>MKRSWF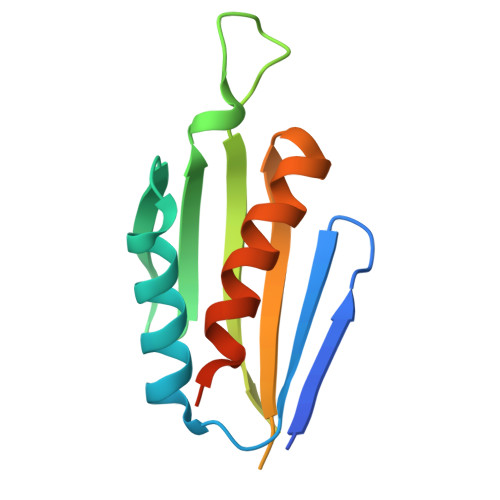GNFISLDKEEQIFLVLKDKPLSSIKADIVHAFLSIPSLSHSVLSQTSFRAEYKASGGPSVFQKPVRFQVDISSSEGPEPSPRRDGSSGGGIYSVTFTLISGPSRRFKRVVETIQAQLLSTHDQLEHHHHHH[2x]>[2x]MGLLSILRKLKSAPDQEVRILLLGLDNAGKTTLLKQLA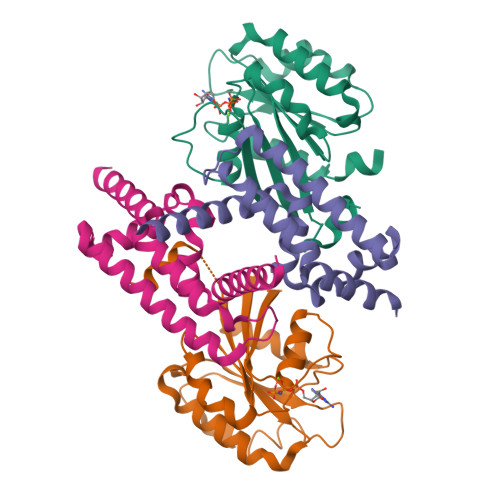SEDISHITPTQGFNIKSVQSQGFKLNVWDIGGQRKIRPYWRSYFENTDILIYVIDSADRKRFEETGQELTELLEEEKLSCVPVLIFANKQDLLTAAPASEIAEGLNLHTIRDRVWQIQSCSALTGEGVQDGMNWVCKNVNAKKKLEHHHHHH;> GPMAAEEEDEVEWVVESIAGFLRGPDWSIPILDFVEQKCEVFDDEEESKLTYTEIHQEYKELVEKLLESYLKEIGINEDQFQEACTSPLAKTRTSQAILQPVLAAEDFTIFKAMMVQKNIEMQLQAIRIIQERNG;> MAAEEEDEVEWVVESIAGFLRGPDWSIPILDFVEQKCEVFDDEEESKLTYTEIHQEYKELVEKLLESYLKEIGINEDQFQEACTSPLAKTRTSQAILQPVLAAEDFTIFKAMMVQKNIEMQLQAIRIIQERNG> GGHNVAWDYDNNVIRGVNLGGWFVLEPYMTPSLFEPFQNGNDQSGVPVDEYHWTQTLGKEAALRILQKHWSTWITEQDFKQISNLGLNFVRIPIGYWAFQLLDNDPYVQGQVQYLEKALGWARKNNIRVWIDLHGAPGSQNGYDNSGLRDSYNFQNGDNTQVTLNVLNTIFKKYGGNEYSDVVIGIELLNEPLGPVLNMDKLKQFFLDGYNSLRQTGSVTPVIIHDAFQVFGYWNNFLTVAEGQWNVVVDHHHYQVYSGGELSRNINDHISVACNWGWDAKKESHWNVAGEWSAALTDCAKWLNGVNRGARYEGAYDNAPYIGSCQPLLDISQWSDEHKTDTRR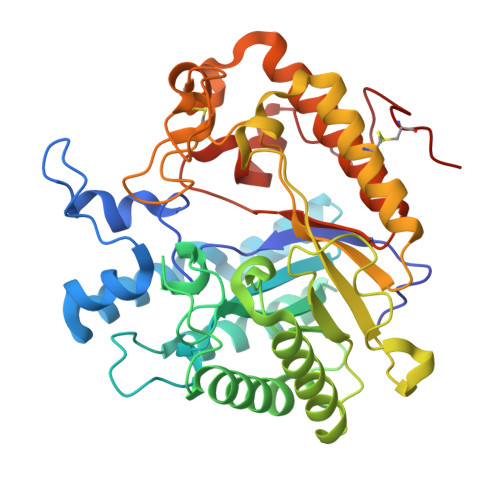YIEAQLDAFEYTGGWVFWSWKTENAPEWSFQTLTYNGLFPQPVTDRQFPNQCGFH> SVNALYDYKFEPKDKVENFHGMQLLYVYWPDHLLFCAPFALLVQPGMTFSALVDEILKPATAAHPDSAKADFLNAEWLLNDEPFT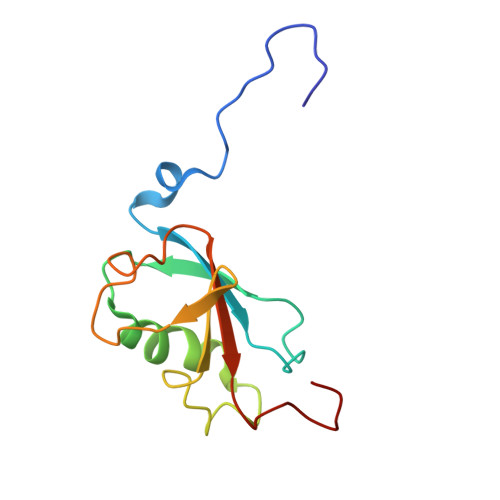PKADASLKEQGIDHKSMLTVTTPGLKGMANAGY[3,5-bis(chloranyl)phenyl]-oxidanyl-oxidanylidene-boron | C6 H4 B 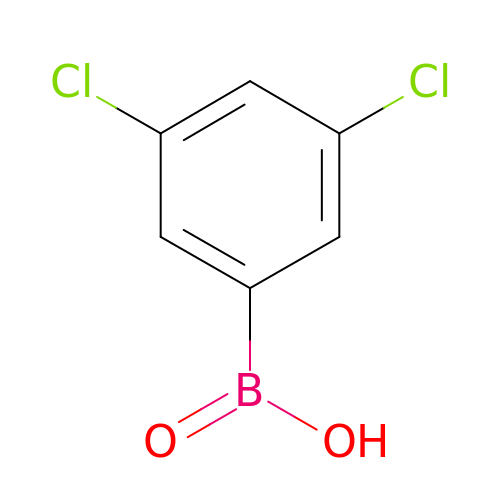Cl2 O2 | QFYDXKOJHIFUIC-UHFFFAOYSA-N> MTFAKIKFSAQIRLETGLHIGGSDAFAAIGAIASPVIKDPITNIPIIPGSSLKGKMRTLLAKVYNEKVAEKPSDDSDILSRLFGNSKDKRFKMGRLIFRDAFLSNADELDSLGVRSYTEVKFENTIDRITAEANPRQIERAIRNSTFDFELIYEITDENE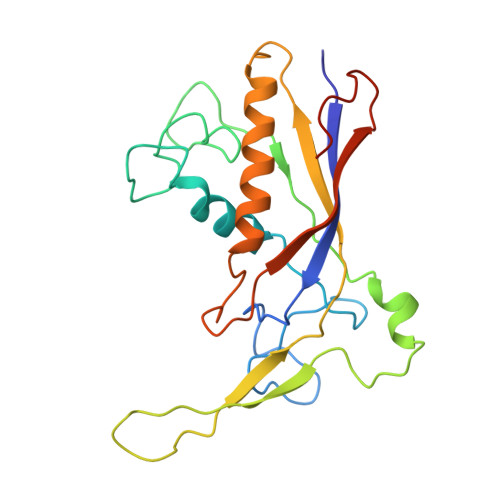NQVEEDFKVIRDGLKLLELDYLGGSGSRGYGKVAFEKLKATTVFGNYDVKTLNELLTAEV>[2x]HMAKHQIGVIGLAVMGKNLALNIESKGYSVAVYNRLREKTDEFLQEAKGKNIVGTYSIEEFVNALEKPRKILLMVKAGAPTDATIEQLKPHLEKGDIVIDGGNTYFKDTQRRNKELAELGIHFIGTGVSGGEEGALKGPSIMPGGQKEAHELVRPIFEAIAAKVDGEPCTTYIGPDGAGHYVKMVHNGIEYGDMQLIAEAYFLLKHVLGMDAAELHEVFADWNKGELNSYLIEITADIFTKIDEETGKPLVDVILDKAGQKGTGKWTSQNALDLGVPLPIITESVFARFLSAMKDERVKASKVLAGPAVKPFEGDRAHFIEAVRRALYMSKICSYAQGFAQMKAASEEYNWNLRYGDIAMIFRGGCIIRAQFLQKIKEAYDRDPALSNLLLDSYFKDIVERYQDALREIVATAAMRGIPVPGSASALAYYDSYRTAVLPANLIQAQRDYFGAHTYERVDKEGIFHTEWLK

Two crystal structures of recombinant Geobacillus stearothermophilus 6-phosphogluconate dehydrogenase (Gs6PDH) in complex with the substrate 6-­phosphogluconate have been determined at medium resolution. Gs6PDH shares significant sequence identity and structural similarity with the enzymes from Lactococcus lactis, sheep liver and the protozoan parasite Trypanosoma brucei, for which a range of structures have previously been reported. Comparisons indicate that amino-acid sequence conservation is more pronounced in the two domains that contribute to the architecture of the active site, namely the N-terminal and C-terminal domains, compared with the central domain, which is primarily involved in the subunit–subunit associations required to form a stable dimer. The high degree of structural similarity, efficient level of expression and straightforward crystallization conditions mean that Gs6PDH may prove to be an appropriate model system for structure-based inhibitor design targeting the enzyme from Trypanosoma species.

Two isomorphous crystal structures were determined. Data set I was obtained from a sample grown in the presence of 6PG and NADP+ and data set II was obtained from crystals grown in the presence of R5P and NADP+. In neither structure was there electron density that could be attributed to NADP+. In structure I, 6PG is present in both active sites of the dimer that constitutes the asymmetric unit. Crystal I was frozen and stored in liquid nitrogen within one week of setting up the crystallization conditions. A pronounced similarity of the two subunits in the asymmetric units of both crystals is observed despite not employing noncrystallographic symmetry restraints during refinement. The overlay of 467 Cα positions of structure I subunit A on subunit B results in an r.m.s.d. of 0.53 Å; for structure II an r.m.s.d. of 0.70 Å is observed from the overlay of 470 Cα atoms. The overlay of the structure I and structure II dimers, 935 Cα atoms, gives an r.m.s.d. of 0.29 Å. The phosphate of 6PG is positioned by accepting hydrogen bonds from Tyr190, Lys260, Arg287 of one subunit and Arg446 of the partner subunit. Ordered water-mediated hydrogen bonds also link the phosphate group to Asn186, Glu189 and Thr262.> GPHNMATLTDRTYLPPLEDCLTGRTVILSWRLVASALEDADLARLTSPALSTFLRDGFVHELLKHPARVFEPKDLKQEFETKTSSIQTVAPGVDTIKKDALWLADAVAINQVAALRIVLIEYQTRAHSHLVLPLSTQDVANIQEAAGVGDAHASSILSLLNPASAVDAETMWCDFETEARRRERILATYLSERRSFTAAVDALVTFLLHSAPGQHKDLDSLRRALLKDAFAFDEDLDVPDRSKLLTMAPTYMNLVEDCIARAQALPAKLGESFKTEAFELDWLRTAITEAVHSLSIAFQALDLDTPYFAPHELLSEWFELMNSSLFLESILGFEVVADLAMPARSLVSAICLKMLNIDRTIQFLHDFDYPDGEEPYLLSSQTLNKIHTAVTNAVNSGVAASLPVAFAWSLIVHQMHLGYQERAERRDLLVNQRAQAGFELEFQPSASTPNRRRRNSAGSIVSLEASPYDDFLREQRLDNDIAPVEQIAMLATSRGQVYQVMSEMALCLGTTHEAAFRPAVGARARLVFQDLLKRSAYLIPYQDEPVFSLLAILATGRQYWDVTDALSASSLNQVYTDMLDDETLFTQFTMQAINRFPYEFNPFSVLCRVLAAALITNKDKADVVTGWLWRTPTLTVDWNPAWDRSYELCFEDENTNSFRLTRDVDLFGSASPARPRHLAAEERFIIPEGTLGRFVTDVGRTARLEFEHSALALLGKRLEVKAAEEICDSGMAPLDVDEQAEAVAMLATVLRAESLKSTAKGGDPEAPLKFLKEASRLLPHNKDILTVISDTIDGLVEKELLELDGPQIAVLASCLQFLHAALAVCPGRVWAYMSRCALIAGDARPGRLSRITGSLDMYAERFDLLSSAVKLFAALIDSAACSAVQRRAGSTALVSVRSAVENPWLGTSEKILSRVALAIAQAALDVYESTTTWRFRSELDRSILVRDVVGLMHKLVVHAHTLSSHLTSTLSPAAAHIISSFLTPPPSASSLRFQPLLGTLLVALITPRATLYPGQSRILAERVTSVLAFCTSLLRAADFLGQTHIPLQTHLFQSACLLARLPAANAVYRAPVLELLRALVEVAGRAANGSGEPPSLLGYLGSHAARSFISLVEGIDKPFGRVEHAVVTWRFFAAVIRNRQQWMAGCLLTGRTPREALKGGGEQKIERKVGEGSVLAAAMERLREVKSLDVQEAVAVMDFVVSAQNYWPWTIFAVRKEKEVVDALRGYVRGLKAPGMVMKTDGAAAAAFQARIAAYVAETFAMQLYHMRQMRQAEKFAGELVADLDYFLREGVMVWGYNASLHGNFARNFAKRFPGVEVDDFKRTMWLPRELGKGYYYALEVAEQMLGFDAGWGGVKQSGFRKEMETANLNLSLVEAQVSLFHAWEYLLLELTLSLLPKKENAAFARQVLQVVEQCLEANQRSQPPENIFVVLGHARAGLALTLLQRLADANQLPRDVTHLLALVSSAIHAVENPFGANDLPYFRTLLKILFVVLRAAKQGTAKPGESNVAITQQVLTILDRVVARCFRALAALVHEQQQNATDGTTTAPEDLALITAILQACLSVPGIEQCQVQVLNIMAAHDVFQVAVALFSWADRLLPANPSPASSSTSTSATNPASGDPVYGELALLFLLELSALPALAEHLACDGLLGHLAAARLAGYMRRTNVGPFAENAGAARCYAIWAKCLLPLLLNILAALGSTVAPEVAWVLNQFPNLLQSSV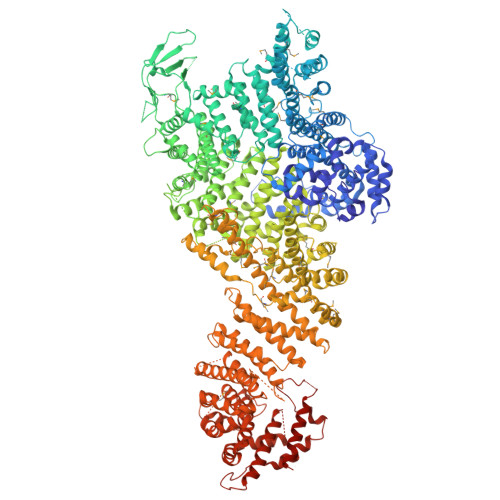ERIEPPGFSRPTLSLASTPPRQKFISLLEISEIHSLALLTRVLAACRAQNARDVPEVTWDGAKVLECVEYWLRGRKVLRERLVPLGPREVEWRGMVATGGVVGVAGDGGEGCENRLEEKAVGLLVGVREVLEGGLEGEGE>[4x]HHHHHHMEPACKYDFATSVLFTEAELHTR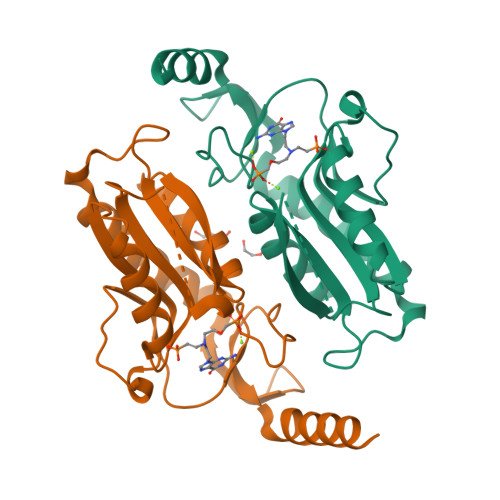MRGVAQRIADDYSNCNLKPLENPLVIVSVLKGSFVFTADMVRILGDFGVPTRVEFLRASSYGHDTKSCGRVDVKADGLCDIRGKHVLVLEDILDTALTLREVVDSLKKSEPASIKTLVAIDKPGGRKIPFTAEYVVADVPNVFVVGYGLDYDQSYREVRDVVILKPSVYETWGKELERRKAAGEAKR>[2x]MLSQIAICIWVESTAILQDCQRALSADRYQLQVCESGEMLLEYAQTHRDQIDCLILVAANPSFRAVVQQLCFEGVVVPAIVVGDRDSEDPDEPAKEQLYHSAELHLGIHQLEQLPYQVDAALAEFLRLAPVETMADHIMLMGANHDPELSSQQRDLAQRLQERLGYLGVYYKRDPDRFLRNLPAYESQKLHQAMQTSYREIVLSYFSPNSNLNQSIDNFVNMAFFADVPVTKVVEIHME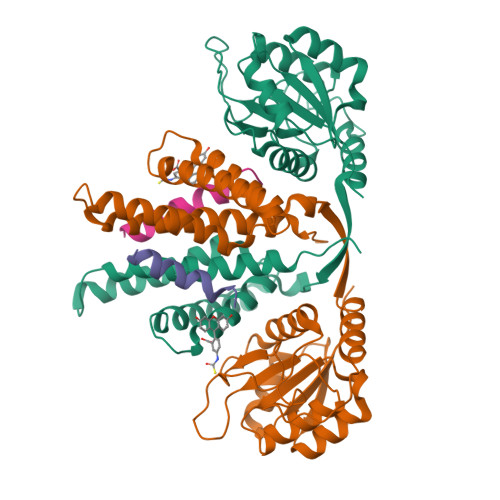LMDEFAKKLRVEGRSEDILLDYRLTLIDVIAHLCEMYRRSIPRETHHHHHH;>DEKSELSRIVRGVQEKGPES[2x]> PKLVTWMNNQRVGELTKLANGAHTFKYAPEWLASRYARPLSLSLPLQRGNITSDAVFNFFDNLLPDSPIVRDRIVKRYHAKSRQPFDLLSEIGRDSVGAVTLIPEDETVTHPIMAWEKLTEARLEEVLTAYKADIPLGMIREENDFRISVAGAQEKTALLRIGNDWCIPKGITPTTHIIKLPIGEIRQPNATLDLSQSVDNEYYCLLLAKEL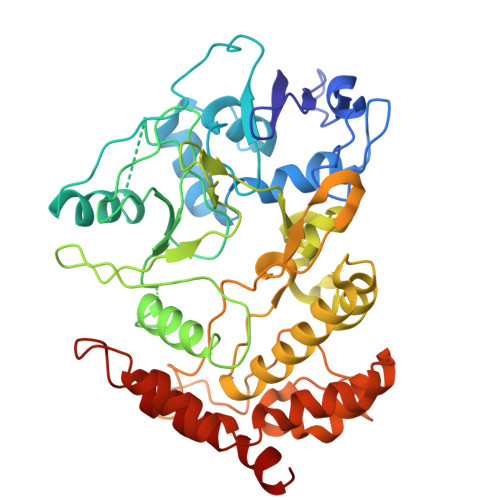GLNVPDAEIIKAGNVRALAVERFDRRWNAERTVLLRLPQEDMCQTFGLPSSVKYESDGGPGIARIMAFLMGSSEALKDRYDFMKFQVFQWLIGATQGHAKNFSVFIQAGGSYRLTPFYDIISAFPVLGGTGIHISDLKLAMGLNASKGKKTAIDKIYPRHFLATAKVLRFPEVQMHEILSDFARMIPAALDNVKTSLPTDFPENVVTAVESNVLRLHGRLSREY1-ethyl-N-(2-fluorophenyl)piperidin-4-amine | C13 H19 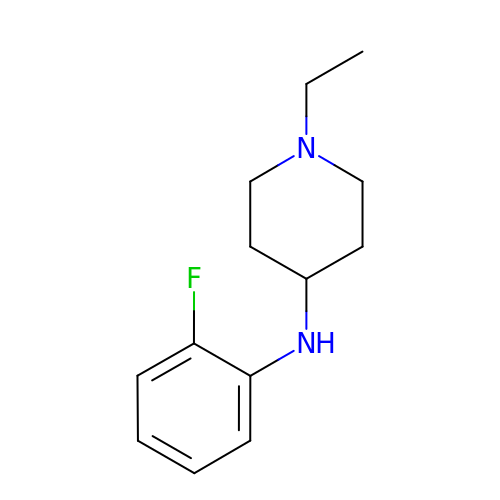F N2 | JXDKAPWBGLJUDX-UHFFFAOYSA-N> ACDYTCGSNCYSSSDVST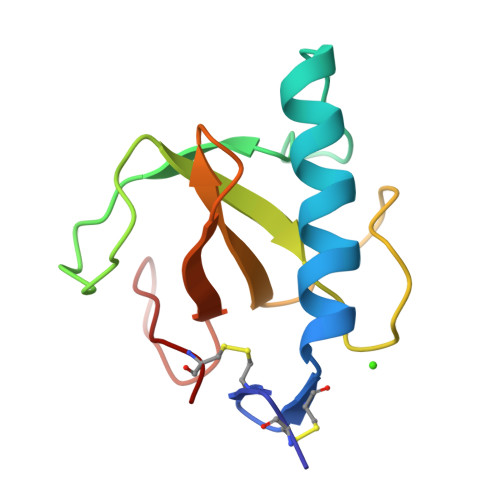AQAAGYKLHEDGETVGSNSYPHKYNNYEGFDFSVSSPYYEWPILSSGDVYSGGSPGADRVVFNENNQLAGVITQTGASGNNFVECT3-[4-(2-hydroxyphenyl)phenyl]-4-oxidanyl-6-oxidanylidene-7H-thieno[2,3-b]pyridine-5-carbonitrile 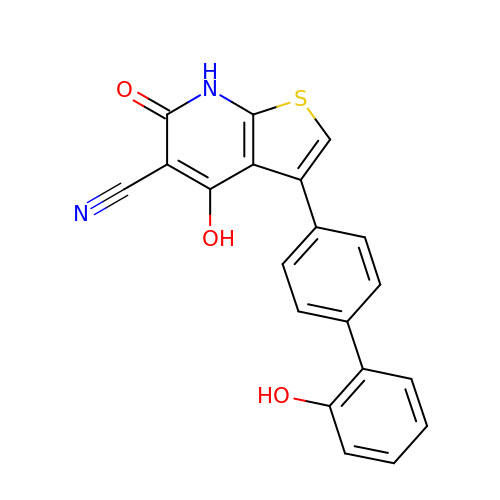| C20 H12 N2 O3 S | CTESJDQKVOEUOY-UHFFFAOYSA-N>[2x]GPMIDLYTAATPNGHKVSIALEEMGLPYTVHALSFDKKEQKAPEFLRINPNGRIPAIVDRSND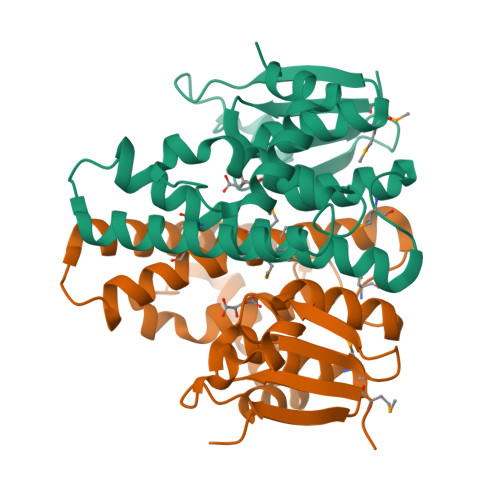DFAVFESGAILVYLAEKTGQLMPTDVKGRSRVIQWLMFQMGGVGPMQGQANVFFRYFPEKLQGAIDRYQHETRRLYEVLDGRLGEAEYLAGDYSIADIATYPWVRIHDWSGVAVDGLDNLQRWIAALEARPAVQRGLLVPRREKEGDDAIRTAQSMLTR> MSGSLREEIRKLAEQLSEKYKDEEIRELAREAAELAEESDDPEVLELAYEALKKGLELEDEEKVKLILLAAVLAARVARGEVPEEKLEIALKALELAEASEDERIIRGALRAALAAARTDDPLALEVVLEALERAQASEDERLIRAILAAAYAFALLAVAGASAERLKEAEAIVKELIAAAEKGASPQELVLLVIEMMVKGMGVTMETHRSGNEVKVVIKGLHESQQEVLLEAVLFAAELMGVRVRIRFKGDTVTIVVRE;> EERKKELAKEVIETAK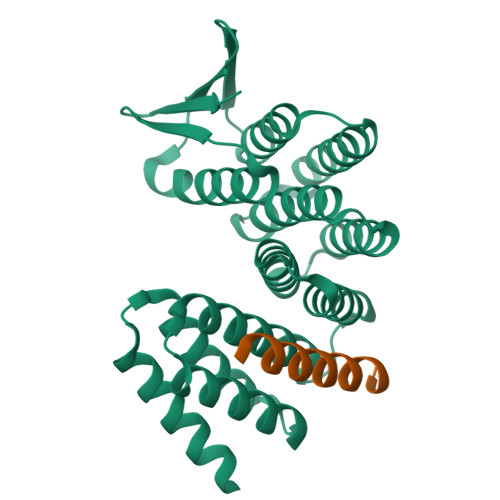KLIEKLAKEE> GSHAAILWNEAKAFIAECYAELGKAEEVADRLDSIKSEIDRTGSYVHTKEELEH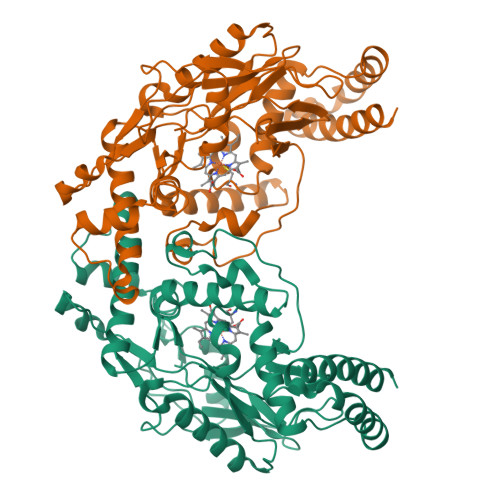GAKMAWRNSNRCIGRLFWNSLNVIDRRDVRTKEDVRDALFHHIETATNNGKIRPSITIFPPEEKGEKQVEIWNHQLIRYAGYEGEAIGDPASRSLTAACEQLGWRGERTDFDLLPLIFRMRGDEQPVWYELPRSLVIEVPITHPDIEAFSDLELKWYGVPIISDMKLEVGGIHYNAAPFNGWYMGTEIGARNLADEKRYDKLKKVASVIGISTNYNTDLWKDQALVELNKAVLYSYKKQGVSIVDHHTAASQFKRFEEQEEEAGRKLTGDWTWLIPPISGAATHIFHRSYDNSIVKPNYFYQDKPYE>[2x]MGSDKIHHHHHHMKEVFDLRGRVALVTGGSRGLGFGIAQGLAEAGCSVVVASRNLEEASEAAQKLTEKYGVETMAFRCDVSNYEEVKKLLEAVKEKFGKLDTVVNAAGINRRHPAEEFPLDEFRQVIEVNLFGTYYVCREAFSLLRESDNPSIINIGSLTVEEVTMPNISAYAASKGGVASLTKALAKE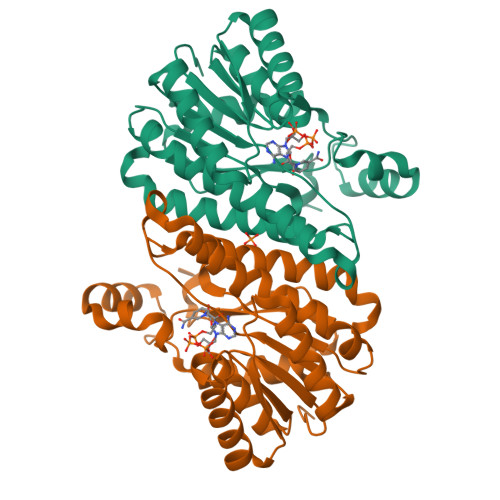WGRYGIRVNVIAPGWYRTKMTEAVFSDPEKLDYMLKRIPLGRTGVPEDLKGVAVFLASEEAKYVTGQIIFVDGGWTAN(5-fluoro-1H-indol-2-yl)[(3R)-1'-[(3R)-piperidin-3-yl]spiro[indole-3,3'-pyrrolidin]-1(2H)-yl]methanone 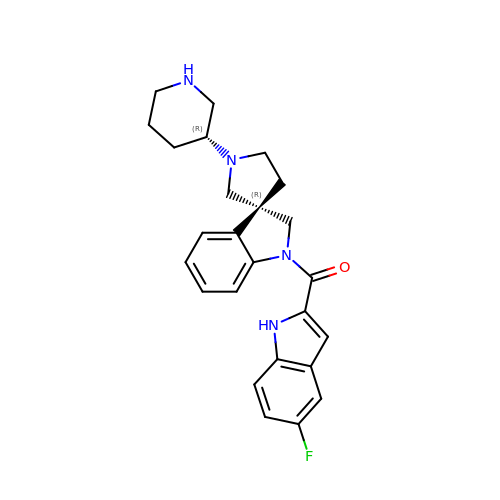| C25 H27 F N4 O | ABNVVKAVWJYHCL-KBMIEXCESA-N>SGSSEELARESAEAAWRLAQASTRATLAMIRGDLKELAEALIELARAVQELARVAKEYGNDELAKTAALLAAHVAMLAIWVLIRAIKEGDDEVRELAKTAIKLASTAAKIVLDALPTAEEVRQITLLAKLAEEA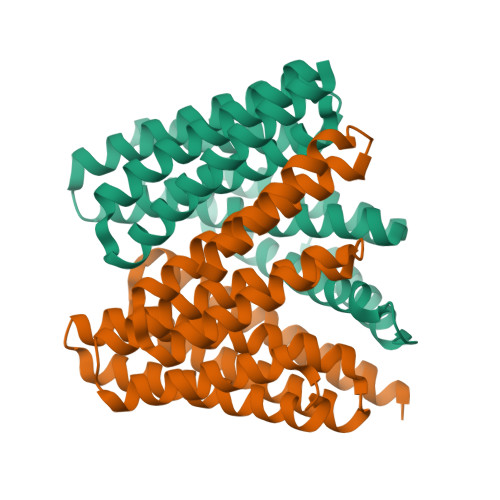ADKKNEDSALAVGIAAIAVIIALWALEAAQKAGIEEAEKGARLLLKLAMDAARKKNPEEALAVLNAALDVSIALQLLQSAKRAGSEETRKLAEEMLRQALERARKKN[2x]>GSHMSQATSQPINFQVQKDGSSEKSHMDDYMQHPGKVIKQNNKYYFQTVLNNASFWKEYKFYNANNQELATTVVNDNKKAD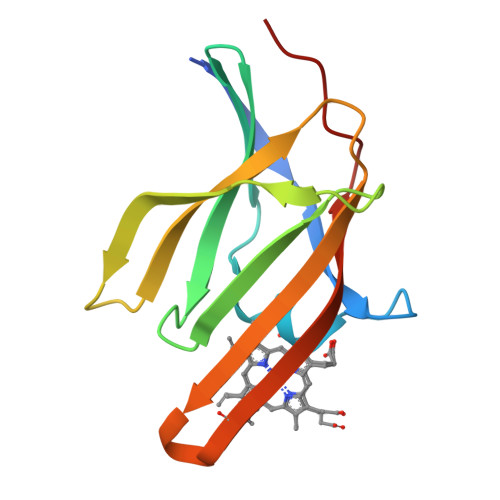TRTINVAVEPGYKSLTTKVHIVVPQINYNHRYTTHLEFEKAIPTLA[4x]>SNANEAQQYYLDADEAEAWIGEQELYVISDEIPKDEEGAIVMLKRHLRQQRAVEDYGRNIKQLASRAQGLLSAGHPEGEQIIRLQGQVDKHYAGLKDVAEERKRKLENMYHLFQLKRETDDLEQWISEKELVASSPEMGQDFDHVTLLRDKFRDFARETGAIGQERVDNVNAFIERLIDAGHSEAATIAEWKDGLNEMWADLLELIDTRMQLLAASYDLHRYFYTGAEILGLIDEKHRELPEDVGLDASTAESFHRVHTAFERDVHLLGVQVQQFQDVATRLQTAYAGEKAEAIQNKEQEVSAAWQALLDACAGRRTQLVDTADKF[2x];>SNATGFLVSFMVDARGGSMRGSRHNGLRVVIPPRTCAAPTRITCRLVKPQKLSTPPPLAEEEGLASRIIALGPTGAQFLSPVIVEIPHFASHGRGDRELVVLRSENGSVWKEHR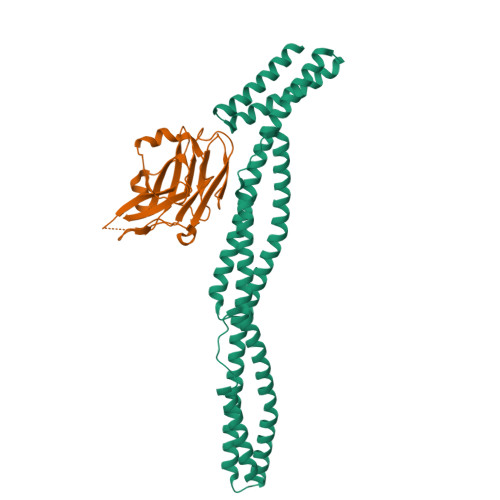SRYGESYLDQILNGMDEELGSLEELEKKRVCRIITTDFPLYFVIMSR[2x]>[2x]MFN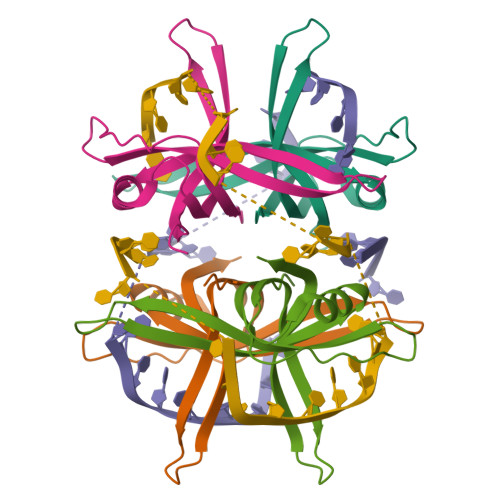KVIMVGRLTRNVELKYLPSGSAAATIGLATSRRFKKQDGTLGEEVCFIDARLFGRTAEIANQYLSKGSSVLIEGRLTYESWMDQTGKKNSRHTITADSLQFMDKKSDNPQANAMQDSIMHENSNNAYPANH>[2x]SNANEDILERSKSTNEIIWGVKYDTRLFGMMDIESRTVQGFDVDIAKAITK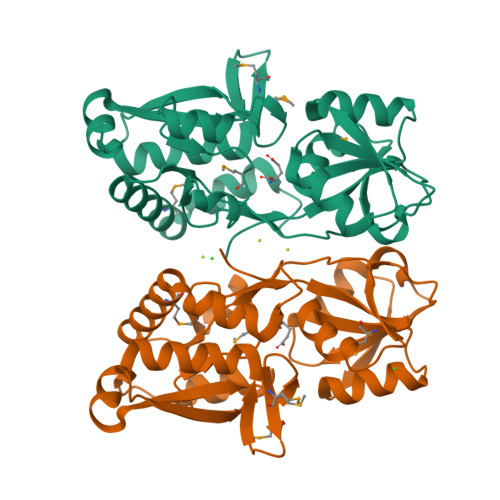KILGDNGKTEFVEVTSKTRIPLLKNGNIDAIIATMTITDERKKQVDFSDVYFDAGQALLVKKGSQIKSVDDLNASTTVLAVKGSTSAANIRQHAPDAKILELENYAEAFTALQSGQGDAMTTDNAILLGIADENPEYELVGGTFTNEPYGIAINKGQENFLKAVNQALEEMHADGTYDKIYQKWFPNETEGKVE> MVFHKIRNEDLIFNESLGQGTFTKIFKGVRREVGDYGQLHETEVLLKVLDKAHRNYSESFFAAASMMSKLSHKHLVLNYGVCFCGDENILVQEFVKFGSLDTYLKKNKNCINILWKLEVAKQLAAAMHF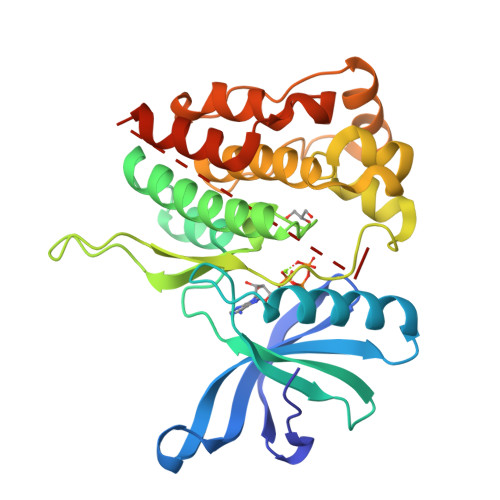LEENTLIHGNVCAKNILLIREEDRKTGNPPFIKLSDPGISITVLPKDILQERIPWVPPECIENPKNLNLATDKWSFGTTLWEICSGGDKPLSALDSQRKLQFYEDRHQLPAPKAAELANLINNCMDYEPDHRPSFRAIIRDLNSLFTPDLVPRGSHHHHHH> MSLNDNNTILGFDVNLICD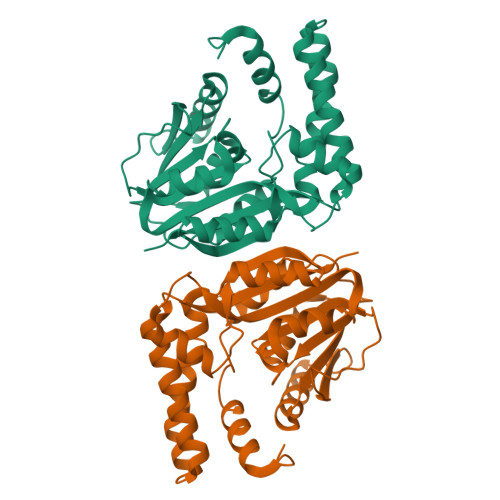FFLNTERQGPGSPEVTLKALSFIDNLTNKSLIADLGCGTGGQTMILAQHVPGKITGIDFFPGFIERFNKNAEKLNLQNRVKGIVGSMDDLSFEKDSLDLIWSEGAIYNIGFERGLKEWRNYLKPGGYLAVSESVWFTDQRPAEIHDFWMSAYTEIDTVPNKVAQIQKAGYIPVATFILPENCWIEHYFAPQAKAEEIFRRKHAGSRIVEELITSNHHEAELYSKYKAYYGYAFFICKKGFSLREGHHHHHH> AIKKDQKAPVVTIFDARGCKDHSNKEYTGAKAGGMEDDQCVKLTMETIKVGDDVAAKVLGECLSELK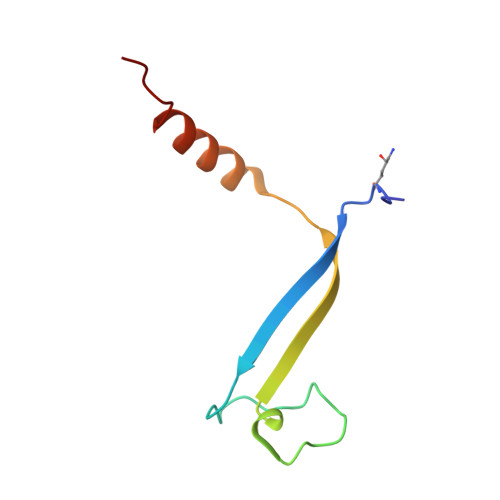SRK2-[2-(hydroxymethyl)-3-{1-methyl-6-oxo-5-[(pyrimidin-4-yl)amino]-1,6-dihydropyridin-3-yl}phenyl]-6,6-dimethyl-3,4,6,7-tetrahydro-2H-cyclopenta[4,5]thieno[2,3-c]pyridin-1(5H)-one 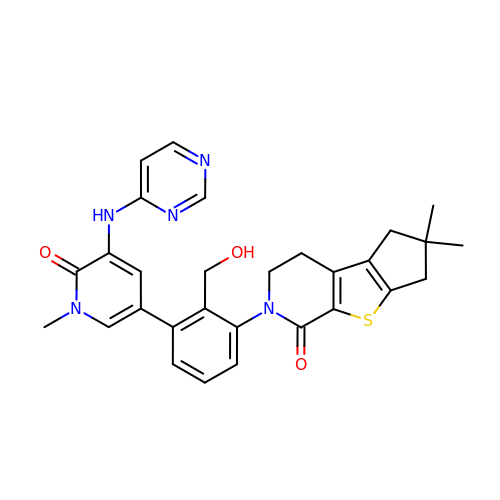| C29 H29 N5 O3 S | QAESSIFTPVEYRY-UHFFFAOYSA-N>[4x]DTLVGRADEKANERHSPQTESMITSIGNPAQVLKVRETFGTWMRESANKSDDRIWVTEHFSGIMVKEFKDLPALLNSSFTLLHLPHYFHGCGHAVYNNSLYYHKGGSNTIVRFEFGKETPQTLKLENALYFDRKYLFANSKTYFNIAVDEKGIWIIYASSVDGSSILVAQLDER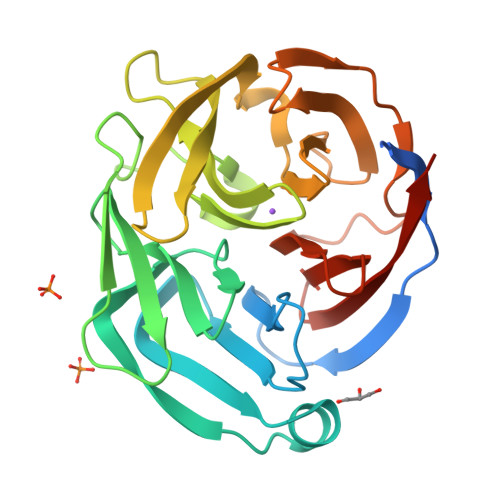TFSVTQHINTTYPKSKAGNAFIARGILYVTDTKDTRVTFAFDLLGGKQINANFDFRMSQSVLAMLSYNMRDQHLYSWEDGHLMLYPVQFLSAASSQR> QDVFLLALGTEPLNCFSQTFEDLTCFWDEEEAAPSGTYQLLYAYRGEKPRACPLYSQSVPTFGTRYVCQFPAQDEVRLFFPLHLWVKNVSLNQTLIQRVLFVD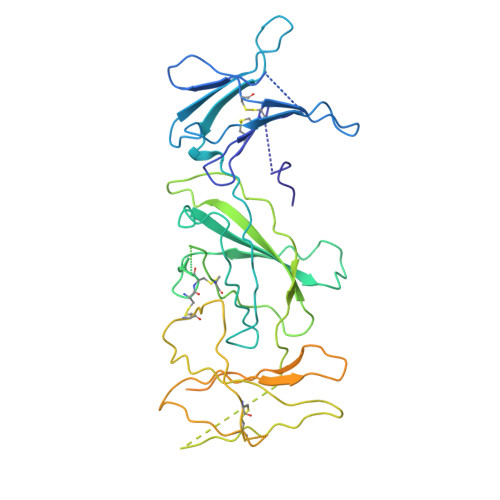SVGLPAPPRVIKARGGSQPGELQIHWEAPAPEISDFLRHELRYGPTDSSNATAPSVIQLLSTETCCPTLWMPNPVPVLDQPPCVHPTASQPHGPAPFLTVKGGSCLVSGLQAGKSYWLQLRSQPDGVSLRGSWGPWSFPVTVDLPGDAVTIGLQCFTLDLKMVTCQWQQQDRTSSQGFFRHSRTRCCPTDRDPTWEKCEEEEPRPGSQPALVSRCHFKSRNDSVIHILVEVTTAQGAVHSYLGSPFWIHQAVLLPTPSLHWREVSSGRLELEWQHQSSWAAQETCYQLRYTGEGREDWKVLEPSLGARGGTLELRPRARYSLQLRARLNGPTYQGPWSAWSPPARVSTGSETAWENLYFQ>GDHYDDELFSDVQDIKTALAKIHEDNQKIISKLESLLLLKGEVESIKKQINRQNISISTLEGHL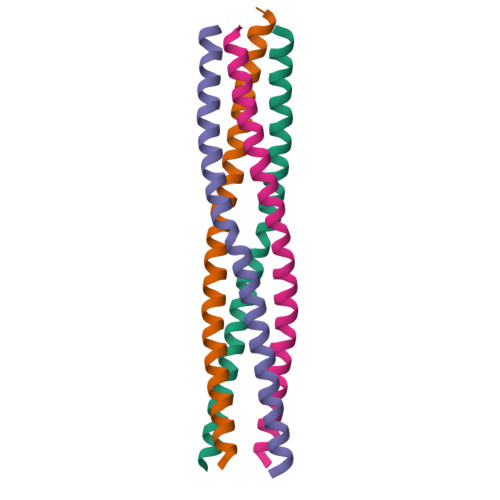SSIMIAIPGLLEHHHHHHHH[8x]>[2x]MRGSHHHHHHGSMPDLLT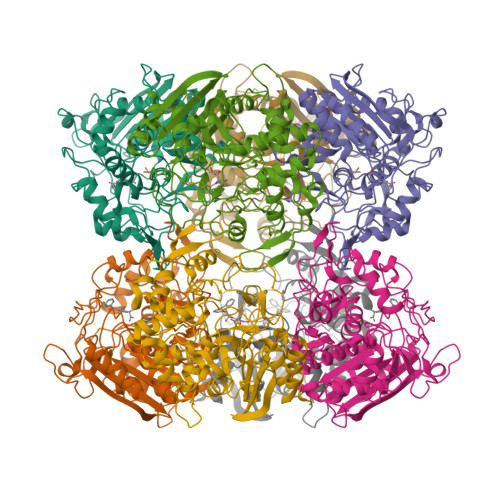NVAENYVNQDLFAGIEWRIDQDGKPIFQGCAGVKDIETRTFIPKNAIYRIYSMTKPIVSFLAMMLIERGVFRLSSPIQNFDPRFKSMKVIDQHAHIEPATALITIEHLLTHQAGFSYDFSLGCPISAHYRDAQLIEDGGRDLTDMMGVLAELPLVFHPGTQWKYSISTDVLAHIIECATGERVDDLLQRLIFDPLDMQDTGFSLPLDGASRLMEVYGMRSLAGLPALKPAPHVLVPADLGSSHPTDDPDFRRGGHGLYSTLDDYMAFANMLLSGQTPEGETLLSPAVLKLALAPRVHFGARGMRINDEPFAGYSWNLLGRVMTDVGAAAYATHLGEFGWSGAAATYFWVDPTKNMTGCVMTQFLGSQHPIGSDMQAAAMSMLG>GSMQNRQVANATKVAVAGASGYAGGEILRLLLGHPAYADGRLRIGALTAATSAGSTLGEHHPHLTPLAHRVVEPTEAAVLGGHDAVFLALPHGHSAVLAQQLSPETLIIDCGADFRLTDAAVWERFYGSSHAGSWPYGLPELPGARDQLRGTRRIAVPGCYPTAALLALFPALAADLIEPAVTVVAVSGTSGAGRAATTDLLGAEVIGSARAYNIAGVHRHTPEIAQGLRAVTDRDVSVSFTPVLIPASRGILATCTARTRSPLSQLR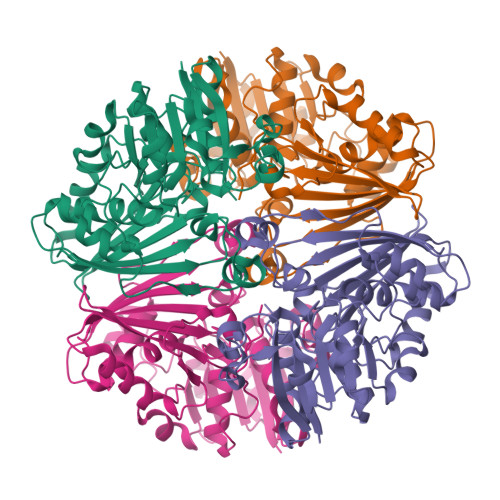AAYEKAYHAEPFIYLMPEGQLPRTGAVIGSNAAHIAVAVDEDAQTFVAIAAIDNLVKGTAGAAVQSMNLALGWPETDGLSVVGVAP[2x]>[2x]MGSSHH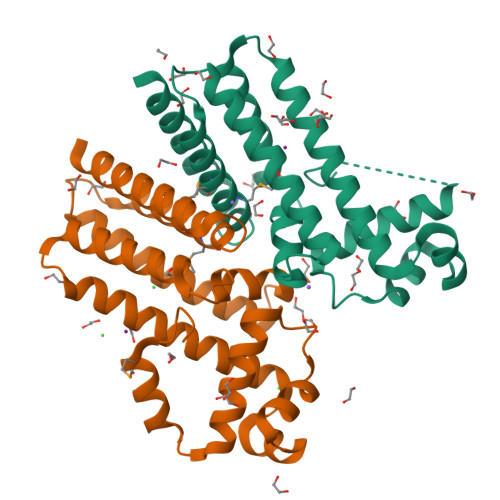HHHHSSGRENLYFQGMSPSTEAAARTPSEARARLLGTATRIFYAEGIHSVGIDRITAEAQVTRATLYRHFSGKDDLILAYLDQADRGIRAQVTAARGSSPAADGQVRAVARSIVDGIRSPGFRGCAFLNAVAEYPDPAHPVHRAVLAHRQWFLDTVTELLAQVGDGDGVAAGRHLVMLRDGAMAAGCLFDPELVSETFLHGVEGVLRDVSEKTSA> GAMGNPLRKFKLVFLGEQSVGKTSLITRFMYDSFDNTYQATIGIDFLSKTMYLEDRTVRLQLWDTAGLERFRSLIPSYIRDSTVAVVVYDITNVNSFQQTTKWIDDVRTERGSDVIIMLVGNKTDLADKRQVSIEEGERKAKELNVMF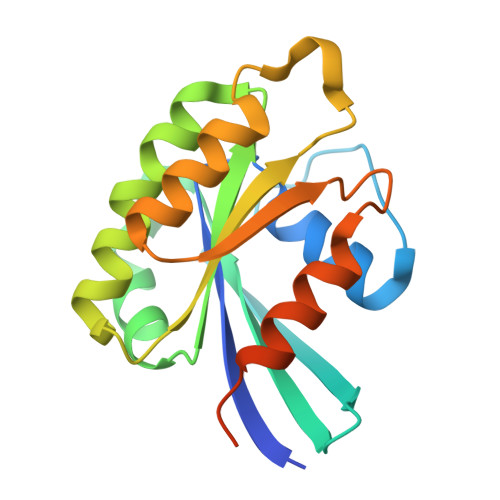IETSAKAGYNVKQLFRRVAAALPGMESTQDRSREDMIDIKLEK>MKTIIINGVQFNTDEDTTILKFARDNNIDISALCFLNNCNNDINKCEICTVEVEGTGLVTACDTLIEDGMIINTNSDAVNEKIKSRISQLLDIHEFKCGPCNRRENCEFLKLVIKYKARASKPFLPKDKTEYVDERSKSLTVDRTKCLLCGRCVNACGKNTETYAMKFLNKNGKTIIGAEDEKCFDDTNCLLCGQCIIACPVAALSEKSHMDRVKNALNAPEKHVIVAMAPSVRASI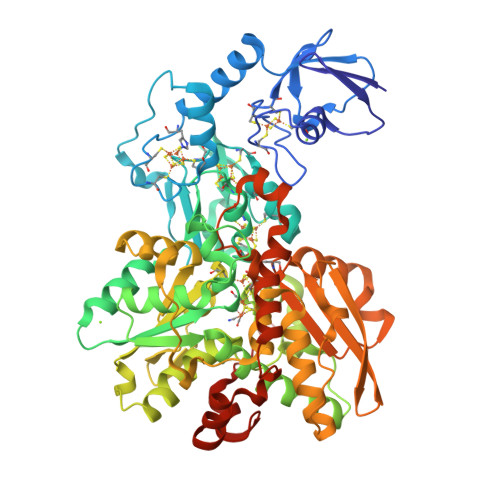GELFNMGFGVDVTGKIYTALRQLGFDKIFDINFGADMTIMEDATELVQRIENNGPFPMFTSCCPGWVRQAENYYPELLNNLSSAKSPQQIFGTASKTYYPSISGLDPKNVFTVTVMPCTSKKFEADRPQMEKDGLRDIDAVITTRELAKMIKDAKIPFAKLEDSEADPAMGEYSGAGAIFGATGGVMEAALRSAKDFAENAELEDIEYKQVRGLNGIKEAEVEINNNKYNVAVINGASNLFKFMKSGMINEKQYHFIEVMACHGGCVNGGGQPHVNPKDLEKVDIKKVRASVLYNQDEHLSKRKSHENTALVKMYQNYFGKPGEGRAHEILHFKYKKSAWSHPQFEK[2x]>[7x]NLIP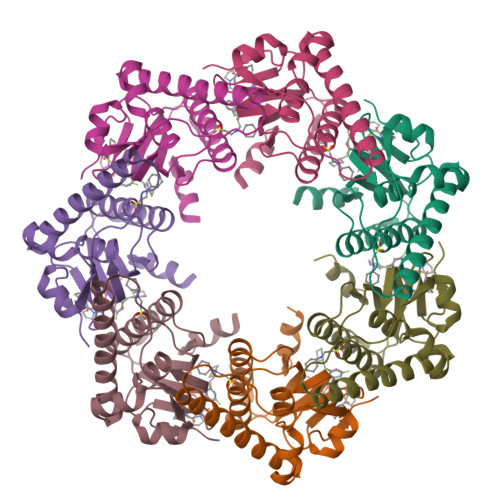TVIEQTNRGERAYDIYSRLLKDRIIMLGSAIDDNVANSIVSQLLFLAAEDPEKEISLYINSPGGSITAGMAIYDTMQFIKPKVSTICIGMAASMGAFLLAAGEKGKRYALPNSEVMIHQPLGGAQGQATEIEIAAKRILLLRDKLNKVLAERTGQPLEVIERDTDRDNFKSAEEALEYGLIDKILTHTEDKKHHH>GEEGNSSELPLSAEDAKKLTELAENVLQGWDVQAEKIDVIQGNQMALVWKVHTDSGAVCLKRIHRPEKKALFSIFAQDYLAKKGMNVPGILPNKKGSLYSKHGSFLFVVYDWIEGRPFELTVKQDLEFIMKGLADFHTASVGYQPPNGVPIFTKLGRWPNHYTKRCKQMETWKLMAEAEKEDPFSQLYLQEIDGFIEDGLRIKDRLLQSTYVPWTEQLKKSPNLCHQDYGTGNTLLGENEQIWVIDLDTVSFDLPIRDLRKMIIPLLDTTGVWDDETFNVMLNAYESRAPLTEEQKQVMFIDMLFPYELYDVIREKYVRKSALPKEELESAFEYERIKANALRQLI[2x]

YtaA (CotI) of B. subtilis is a member of a family of proteins specific to the phylum Firmicutes, which are implicated in spore formation and often form part of the spore coat. The BSKs constitute a new family within the CAK kinases. CAKs adopt a protein kinase-like (PKL) fold, with distinctive CAK-specific structural elements. They usually phosphorylate small molecules, and are named for the choline and aminoglycoside kinase members, which were the first structures to be described.

The crystal structure of YtaA, at 2.5 Å resolution, has an overall similarity to previously determined CAK structures. YtaA contains the PKL bilobed fold, with a smaller, mostly β-stranded N-terminal lobe, and a larger, mostly α-helical C-terminal lobe.12 The electron density indicated that a molecule containing an adenosine moiety was bound in the interlobe cleft, where the adenosine moieties of ATP/ADP are found in other PKL structures. This molecule was present due to copurification with YtaA; it was not provided in the crystallization conditions (see “Materials and Methods” section). We therefore modeled the ligand as adenosine. However, the two primary adenosine interacting residues, W123YtaA and I256YtaA, are conserved in most putatively active BSKs, suggesting the observed interactions are both relevant and indicative of a family-wide pattern. In contrast to other CAKs, YtaA retains the Lys (K72YtaA), but completely lacks the Glu partner, replacing it with S84YtaA, which does not form an analogous interaction. The missing Glu may be functionally replaced by D259YtaA in the Dxe motif (DLD in YtaA). The remaining active site residues, which are required for metal binding and catalysis, are conserved in YtaA (as in APH and ChoK), indicating that this protein is very likely to be catalytically active. Remarkably, the electron density maps for the YtaA structure show additional density for an unknown ligand in this region. However, it is unlikely that this ligand could be the biological substrate of YtaA: it is distant from the key active site residue D239YtaA (D166PKA), which directly coordinates the substrate hydroxyl group.> GPMTARAVRGTKDLFGKELRMHQRIVATARKVLEAAGALELVTPIFEETQVFEKGVGAATDIVRKEMFTFQDRGGRSLTLRPEGTAAMVRAYLEHGMKVWPQPVRLWMAGPMFRAERPQKGRYRQFHQVNYEALGSENPILDAEAVVLLYECLKELGLRRLKVKLSSVGDPEDRARYNAYLREVLSPHREALSEDSKERLELNPMRILDSKSERDQALLKELGVRPMLDFLGEEARAHLKEVERHLERLSVPYELEPALVRGLDYYVRTAFEVHHEEIGAQSALGGGGRYDGLSELLGGPRVPG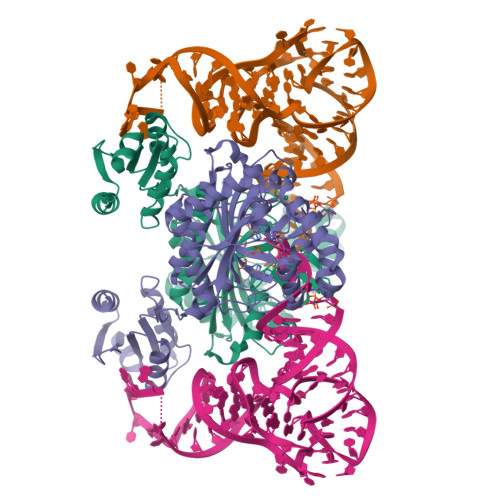VGFAFGVERVALALEAEGFGLPEEKGPDLYLIPLTEEAVAEAFYLAEALRPRLRAEYALAPRKPAKGLEEALKRGAAFAGFLGEDELRAGEVTLKRLATGEQVRLSREEVPGYLLQALG Calreticulin (CRT) is a 46 kDa soluble multifunctional protein that was initially identified as an endoplasmic reticulum (ER) chaperone for monoglycosylated proteins and is also involved in Ca2+ regulation. Similar to its ER membrane homologue calnexin (CNX) ectodomain, CRT is composed of a globular domain, into which a flexible arm-like P (proline-rich) domain is inserted. The globular domain is made up of seven concave and six convex β-sheets forming a legume lectin fold. We have investigated the CRTs of two distinct parasites, Trypanosoma cruzi (TcCRT) and Entamoeba histolytica (EhCRT), for which a pathogenic role has been proposed.

E. histolytica is the causative agent of amoebiasis, a disease mainly characterized by dysentery that leads to about 100 000 deaths per year. During this process, EhCRT is exported from the ER to the phagolysosomal cupule, where it favours the phagocytosis process in a way similar to that described for human CRT on the surface of macrophages during the clearance of apoptotic cells. A similar EhCRT construct was then produced and beautiful crystals were obtained.

>MSAKVYFHETFENRDKWIDSTSSGKALGPFKIVSGKWYGDANNKGLQTSEDNKFYIAAAKLDEEFSNKDKNLIVQYNLKFEQGIDCGGGYIKLLPKKSIESEEKFTPESEYNIMFGPDVCGGSKRTHVIMNYKGKNNLIRKEIKCESDDISHLYTLIIRPNNTYVVKIDGVEKQEGKFDEDWDMLAPKEIDDGSGIANPDYVYDPELYKYDSFAYIGIDVWQVKAGTIYDDILITDDIEEAEKEAKVILERNAAEKKMRDEIKEAENGHHHHHH[2x]N-(3-methyl-5-sulfamoyl-1,3,4-thiadiazol-2(3H)-ylidene)acetamide | C5 H8 N4 O3 S2 | 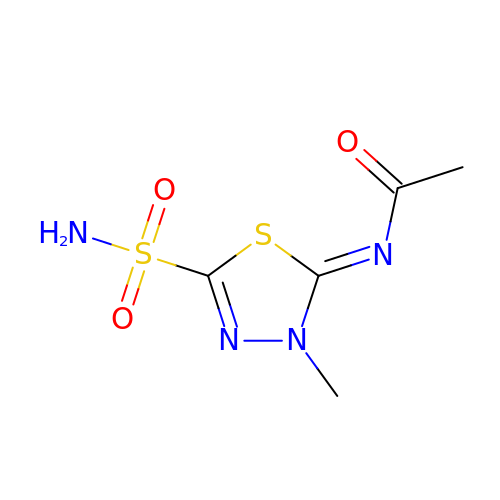FLOSMHQXBMRNHR-DAXSKMNVSA-N> MQVLNTKSETKQENEGSQPPYIQERLKSLNDIETQLCSMLQEASQVTFIFGELKRGNESVKPQFE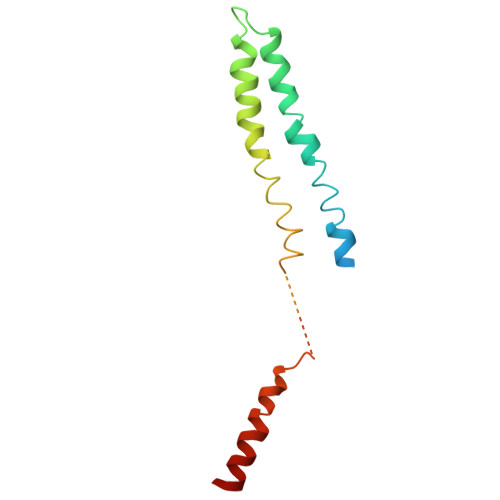NHVKQFYERLDKSTTQLRKEIQLLDENVGTRLLPINVNKKALGQDTEKMEEQLDLLSAILDPSKSK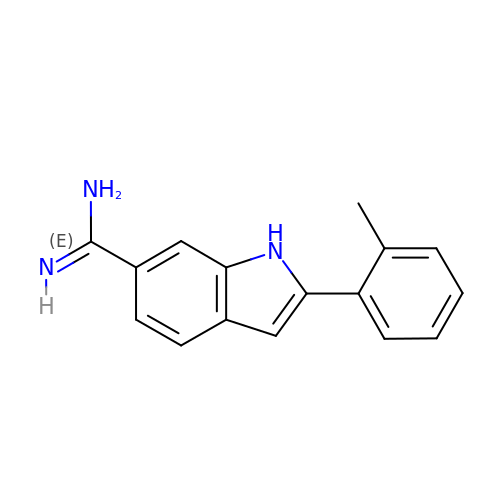2-(2-METHYLPHENYL)-1H-INDOLE-6-CARBOXIMIDAMIDE | C16 H15 N3 | ZRYXDGAKQGRHFG-UHFFFAOYSA-N> UCCCAGUCCACCGU;> CGGUGAGAAGGG;> GGCAGAGAAACACACGA;> UCGUGGUAC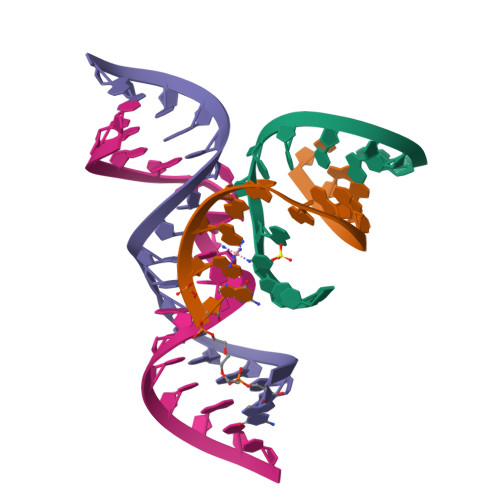AUUACCUGCC> MSYPLSKFHFSVEWGGTKIGFTEVSGLDLETEIIEYRHGASPEYSKIKMPGMQKF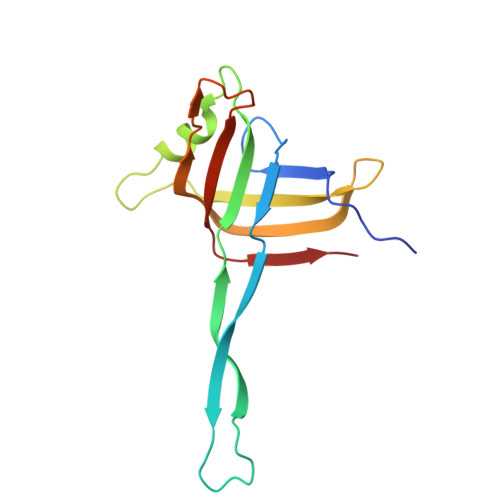SNITLKRGTFKSDNEYFQWYNTINLNKVERRDLTISLLNEEHEPVVTWKVKNAWPLKVQSTDLKGDGNEVAIESMELAHEGLVIQNE> GPSPKANAKLEKVPSGNAESTPVLTLQNRWAYSARDEKLAWDSAARDEKLELTEPAGLIVQFIGENSKHRSVRAKLPIPKGNSGIFYYEVTISGDGDAIYIGLATEQMPLRDTHVGYNEGTYGYGSSGKFWGHEVGGCSHWGNERPYIDGQPKFDRNNIIGCGVNLKTRQIIYTHNGRPLETTGLLVAESAAELYPCVSLFTSGNEIEANFGTKPFKFNIAEG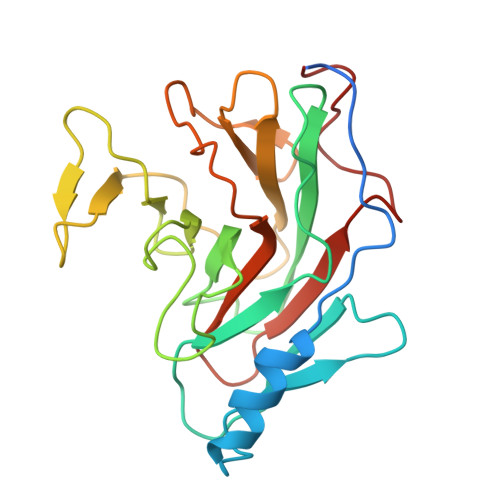I> MSDNLTELSQQLHDASEKKQLTAIAALAEMGEGGQGILLDYLAKNVPLEKPVLAVGNVYQTLRNLEQETITTQLQRNYPTGIFPLQSAQGIDYLPLQEALGSQDFETADEITRDKLCELAGPGASQRQWLYFTEVEKFPALDLHTINALWWLHSNGNFGFSVQRRLWLASGKEFTKLWPKIGWKSGNVWTRWPKGFTWDLSAPQGHLPLLNQLRGVRVAESLYRHPVWSQYGW

Analysis of the plastid-to-nucleus signaling activity of Mg-Proto in Arabidopsis thaliana led to the discovery of GUN4, a novel porphyrin-binding protein that also dramatically enhances the activity of Mg-chelatase, the enzyme that synthesizes Mg-Proto. Although GUN4 is not essential for Mg-Proto synthesis in vitro or in Arabidopsis, GUN4 is required for chlorophyll accumulation in Arabidopsis under normal growth conditions, GUN4 binds porphyrins in vitro, and GUN4 stimulates Mg-chelatase in vitro. Here we report a 1.78-Å resolution crystal structure of Synechocystis GUN4, in which the porphyrin-binding domain adopts a unique three dimensional fold with a “cupped hand” shape. Biophysical and biochemical data support a model wherein the hydrophobic “greasy palm” of the GUN4 core domain, formed by helices that comprise the fingers of the “cupped hand,” wrap around the porphyrin molecule, potentially shielding it from the bulk solvent of the plant or bacterial cell.

To better understand the porphyrin-binding mechanism and Mg-chelatase stimulatory activity of GUN4, we determined the crystal structure of a GUN4 homolog from the model cyanobacterium Synechocystis sp. PCC 6803 (hereafter referred to as Synechocystis 6803) and refined the three-dimensional model to 1.78 Å resolution. The crystallized protein (residues 1–233) comprises the entire Synechocystis GUN4 (SynGUN4) protein. The SynGUN4 structure was solved by multiple isomorphous replacement using crystals soaked with methyl mercury (II) chloride (Hg) and potassium tetrachloroplatinate II-containing compounds. The crystal structure of SynGUN4 reveals a two-domain protein linked by a 12-residue loop. The C-terminal domain, which we refer to herein as the GUN4 core domain, is the conserved domain among all GUN4 family members. The C-terminal domain of SynGUN4, the GUN4 core domain, appears to have no currently identified structural homologs, as indicated by a lack of any structural matches from a search of the DALI server. The helices adopt a concave shell shape resembling a “cupped hand” on one side of the domain, with the back of the “hand” facing toward the N-terminal helical bundle. The buried surface within the concave section of the “cupped hand” is highly hydrophobic. In total, this structural design forms a cavity that is hydrophobic in nature with a volume of about 5,000 Å3. Taken together, the NMR data and the crystal structure strongly suggest that the porphyrin binding region lies within the pocket formed at the intersection of the α6/α7 loop and the “greasy palm” of the GUN4 core domain's “cupped hand” region.~{N}-[3-[(4~{R},5~{R},6~{S})-2-azanyl-6-[1,1-bis(fluoranyl)ethyl]-5-fluoranyl-4-methyl-5,6-dihydro-1,3-oxazin-4-yl]-4-fluoranyl-phenyl]-5-(fluoranylmethoxy)pyrazine-2-carboxamide 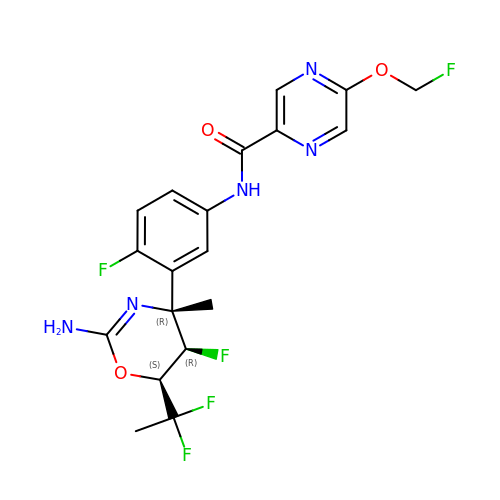| C19 H18 F5 N5 O3 | DKIWJWSKVCKJPV-RLFYNMQTSA-N>VSHVQSSASVPGLIELLESNTIFGNEAELLEKEGLSINYPNCRSWHLGVETSNIINFDTVPANCKAYVEDYLITSKQYQYDSKTVNKEAYFYAKGLALKNDTVNVWIFDLDDTLLSSIPYYAKYGYGTENTAPGAYWSWLESGESTPGLPETLHLYENLLELGIEPIIISDRWKKLSEVTVENLKAVGVTKWKHLILKPNGSKLTQVVYKSKVRNSLVKKGYNIVGNIGDQWADLVEDTPGRVFKLPNPLYYVPSLEHHHHHH[2x]

Arabidopsis thaliana vegetative storage proteins, VSP1 and VSP2, are acid phosphatases and belong to the haloacid dehalogenase (HAD) superfamily. In addition to their potential nutrient storage function, they were thought to be involved in plant defense and flower development. The acid phosphatase activities of these two enzymes require divalent metal such as magnesium ion. Based on protein sequence motif analysis, Arabidopsis VSP1 and VSP2 are classified as acid phosphatases of the haloacid dehalogenase (HAD) superfamily.

In the current study, we presented the crystal structure of recombinant VSP1 at 1.8 Å resolution via the selenomethionine single-wavelength anomalous diffraction (SAD). VSP1 crystallized in space group C2 with two monomers per asymmetric unit. Like most HAD superfamily members, VSP1 structure possessed a two-domain architecture, with a α/β core Rossmanoid domain and a smaller α-helical domain. The size and location of the cap domain suggests that VSP1 belongs to the classical C1 cap type of the HAD superfamily. Consistent with the known members of the HAD superfamily, the active site of VSP1 is located in the cleft between the core and cap domain. Based on the sequence alignment and structure comparison, the four conserved aspartate residues in VSP1 are Asp124, 126, 245 and 249. In addition, a magnesium ion is located at the catalytic center, coordinated by the carbonyl oxygen of Asp126, the carboxyl oxygens of Asp124 and Asp 245, the hydroxyl oxygen of Tyr266 and three water molecules. Recombinant VSP1 is a dimeric enzyme in solution based on the result of gel filtration chromatography, and this was further confirmed by X-ray crystallography. The dimer interface is built by residues from both core domain and cap domain. In VSP1 structure, the intersubunit surface is located away from the active site and seems not involved in the stability of catalytic site and substrate recognition.>[3x]MAHHHHHHMPDTSDPRPTILLVGASRGLGHAMAAE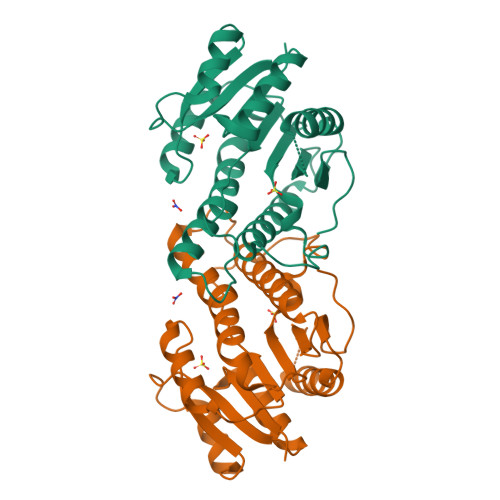FLKRGWDVVGTVRADRGRTPLHALAEAYPDRLRIETLDITQPEQIRALAARLSGRVFDILFVNAGTTNPDPTQTIGEVSTDDFVDLMITNALSPMRVVETLAGLVPRDGLIGIMSSGQGSIADNESGQRELYRGSKAALNQFMRSFAARHAQTPLAMVLIAPGWVRTELGGPDARLSIDESVPGVVDVLLAKRGRAGLEYLDYRGRTVRW>[2x]MVVTRIAPSPTGDPHVGTAYIALFNYAWARRNGGRFIVRIEDTDRARYVPGAEERILAALKWLGLSYDEGPDVGGPHGPYRQSERLPLYQKYAEELLKRGWAYRAFETPEELEQIRKEKGGYDGRARNIPPEEAEERARRGEPHVIRL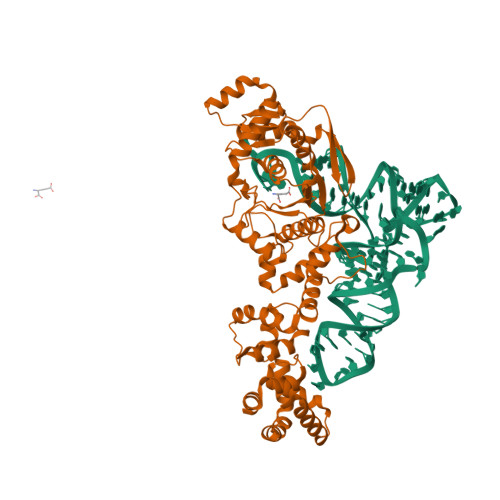KVPRPGTTEVKDELRGVVVYDNQEIPDVVLLKSDGYPTYHLANVVDDHLMGVTDVIRAEEWLVSTPIHVLLYRAFGWEAPRFYHMPLLRNPDKTKISKRKSHTSLDWYKAEGFLPEALRNYLCLMGFSMPDGREIFTLEEFIQAFTWERVSLGGPVFDLEKLRWMNGKYIREVLSLEEVAERVKPFLREAGLSWESEAYLRRAVELMRPRFDTLKEFPEKARYLFTEDYPVSEKAQRKLEEGLPLLKELYPRLRAQEEWTEAALEALLRGFAAEKGVKLGQVAQPLRAALTGSLETPGLFEILALLGKERALRRLERALA>MRGLSRRVQAMKPSATVAVNAKALELRRQGVDLVALTAGEPDFDTPEHVKEAARRALAQGKTKYAPPAGIPELREALAEKFRRENGLSVTPEETIVTVGGSQALFNLFQAILDPGDEVIVLSPYWVSYPEMVRFAGGVVVEVETLPEEGFVPDPERVRRAITPRTKALVVNSPNNP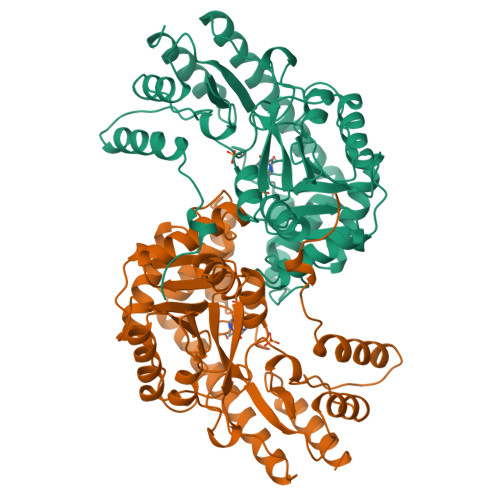TGAVYPKEVLEALARLAVEHDFYLVSDEIYEHLLYEGEHFSPGRVAPEHTLTVNGAAKAFAMTGWRIGYACGPKEVIKAMASVSSQSTTSPDTIAQWATLEALTNQEASRAFVEMAREAYRRRRDLLLEGLTALGLKAVRPSGAFYVLMDTSPIAPDEVRAAERLLEAGVAVVPGTDFAAFGHVRLSYATSEENLRKALERFARVLGRA[2x]> GSMKVKVAINGFGRIGRMVFRKAMLDDQIQVVAINASYSAETLAHLIKYDTIHGRYDKEVVAGEDSLIVNGKKVLLLNSRDPKQLPWREYDIDIVVEATGKFNAKDKAMGHIEAGAKKVILTAPGKNEDVTIVMGVNEDQFDAERHVIISNASCTTNCLAPVVKVLDEEFGIESGLMTTVHAYTNDQKNIDNPHKDLRRARACGESIIPTTTGAAKALSLVLPHLKGKLHGLALRVPVPNVSLV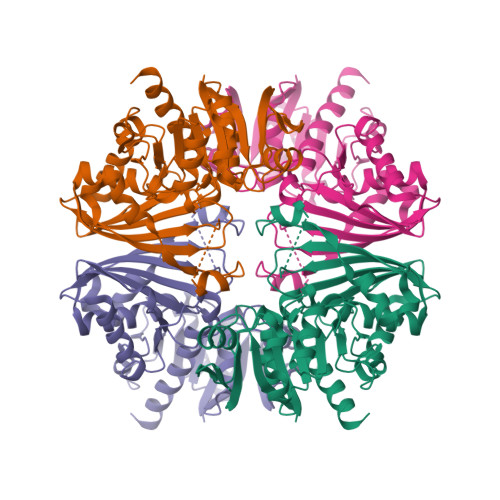DLVVDLKTDVTAEEVNEAFKRAAKTSMYGVLDYSDEPLVSTDYNTNPHSAVIDGLTTMVMEDRKVKVLAWYDNEWGYSCRVVDLIRHVAARMKHPSAV>[2x]GMARRDISGAVDFAYLEGFAAGDFAVVDEVLALFREQAALWAPML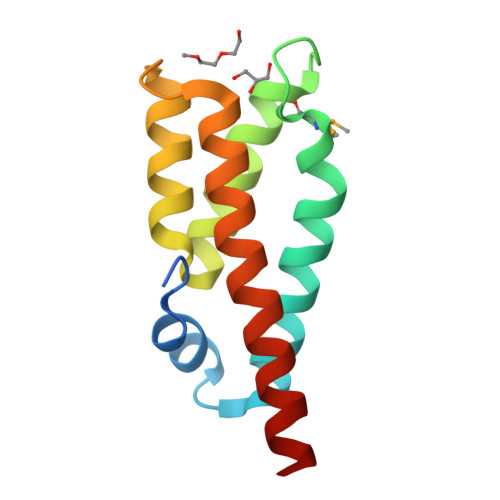DPTHPGWKDAVHTVKGAARGVGAFNLGEVCERCEAGQESLEGVRTALDAALLDIAAYAHEQALRSLKG> MKQILDSARNYLKNNSRIKTASLISLELPGSTGTSTAFIYLTDYFRDVIYNGILYQAGKVKSISPHKQNRDLSIGSLSFTITGTAQDEVLKLVQNGVSFLDRTVSIHQAIITEDGSILPVDPDTNGPLLYFRGRITGGGIKDNISTSGVGTSTITWNCSNQFYDFDRVNGRYTDDASHRGLEVVAGQLLPSNGAKRLEYQEDYGFFHANKSISILAKYQVQEERYKLKSKKKLFGLSRSYSLKKYYETVTKEVDIDFNLAAKYIPVVYGVQKIPGIPIFADTELHNPNIVYVVYAFAEGEIDGFLDFSFGDNPMICVDANDSSARTCFGTKKIVGDTMQRIASGISSSSPSVHGQEYRYNDGNGDIRIWTYHGKSNQTASDVLVNIARNRGFYLQNMNGNGPEYWDARYKLLDTAYAVVRFTINENRTEIPEVSAEIQGKKVKVYHSDGRVTANSTSLNGIWQTLDYLTSDRYGANITIDQFPLQQLIQEAAILDIIDESYQVSWQPYWRYVGWTNPLAENRQIVQMNTILDTSESVFKNVQGLLESYGGAINNLSGQYRVTVEKYSNTPLEINFLDTYGDLELSDTTGRNKFNSVQASIVDPALSWKTNSITFYNSNYKEQDKNLDKKLQLSFANITNYYTARSFADRELKKSRYSRTLSFSLPYQFIGIEPNDAIAFTYDRYGWDRKYFLVDEVENSREGKINVTLQEYGEDVFINSGQVDNSGNDIPDISNNVLPPRDFKYTPTPGGLVGSIGKNGELSWLPSLTNNVVYYSIVHSGHAEPYIVQQLETNPNERMIQEIIGEPAGLAIFEIRAVDINGRRSSPVTLSIELNSAKNLSVVSNFRVTNTASGDVTEFVGPDVKLAWDRIPEEDIIESIFYTLEIHDPQNRMLRSVRIENQYTYDYLLTYNKADFALQNSDALGINRKLYFRIRAEGDDGEQSVEWASI;>MRLPDPYTNPELSGLGFESVNLIDNDPVIRDELPNGKVNEVKVSAQYWGINISYPELFPDEYSVLDAFILEYKRTGGYIDVILPQYEAFRVRGNTNLVNIPAGQKGSNITMDTQGVLTGIPKPGDLFKLSNHPKVYKITSFNRSGNSWSINVYPDLFITTTGAEKPVFNGILFRTKLMNGDAFGSTLNNNGTYSGISLNLRESL[2x];> MYYSLMRESKVIVEYDGRAFHFDALSNYDVQTSYEEFKTLRRTIHRRTNYADSVINAQTPSSISLAINFSNTLTEANFFEWLGFDRKGNTFLLPLYSNNIEPIMFNIYIVNKDNNCVYFENCYVSTVDFSLDKNIPILNVGIESGKFSEVSTYREAASIIQGEAMSYSPVIVSTNGNILPGLISASLSFQQQCSWREDKSVFDINKIYNNKRAYVNEMNASATISLYYLKRFAGDMVYNIEPETDVPLNIRNNNISIDFPLARISKRLNFSDVYKVEWDIIPTASSDPVRIDFFGEIKND;>MSTENRVIDIVVDEKVPYGLIMQFMDVDDSVYPPSEIPVNLTGYSLRGTIKSSLDENAETLASFTTSIIDAAQGAAAISLSVADVTNIGEKASKERDKYNPRQRFAGYYDILMTRDVIGSEVSSFRIMEGKVYISDGVTQ[4x];>MALKTKIIVQQILNIDDTTTTASKYPKYTVVLGN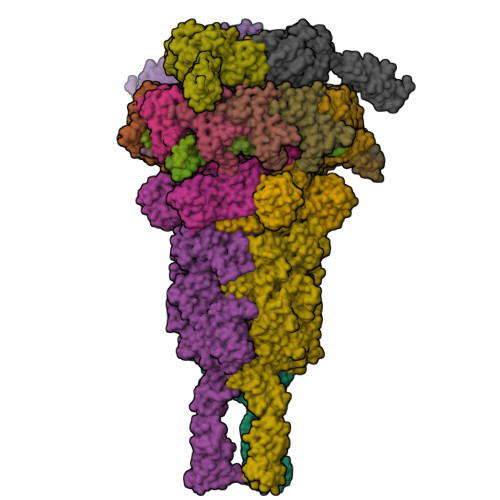SISSITAGELTAAVEASAGSAAAAKGSEIAAKESELNAKDSENEAAISAGASEESASQSAASAAESERQAGLSKGSADNSAASAQESEGFRDSAELAAQNAEQSRLLAEQAKTAAQQAQTAAEAAKTGAETAKDGADAAATTAGEHAAAARQSELNAKISETNAAGSATEAGDKAIDATTEADRAKAEADRATQIVDSKLDKVDISGFIKVYKTKAEADADVVNRVLDEKVLVWNQTNSKYGWYKVAGTAETPVLELVETEQKLTSVNNVRADDAGNVQITLPGGNPSLWLGEVTWFPYDKDSGVGYPGVLPADGREVLRVDYPDTWEAIEAGLIPSVSEAEWQAGASLYFSTGDGSTTFRLPDMMQGQAFRAPTKGEEDAGVIKDQIPYVVTVNGISPDAITGNVEIDTSLQGTVSINQGGTGATTKEDARIALELYSTTEVDSALADKADIATTYTKTEVDSALADKADIATTYTKVEVDSALADAKTQSDTDYLLKANNLSDLADRAAAWLNVRPIGSTPLAGDPVGDYDAVTKRWVENKINTGTVGPTMNGVMNYGVGDFHLRDSRAYIQPYEVVSDGQLLNRADWPELWAYAQMLSPISDADWLADPTKRGQYSLGDGSTTFRVPDRNGVQTGSISALFGRGDGGASSTGGTILDSAAPNITGSFGRLVYASTGTIYEANTGTGAFSAVLSQAKYKRLSEISAADGTAATYPSGFEFFASNSSPVYGRGSTEVRPKAFTGVWVIRASGGFVAANTSWSVINGDATRPADGTTADGGEIISRYNVNGVREAQMSWRIRAQIGAEHYARLNVYNATANRTAVYDFNDLGTFSAENLHSKGAIYSDGNLTIQNQGWPGINFKSNRYNTPATQIGGSTIIEVSGTDGNVSGVNLIRRRGDGNQAGQIIVSFPTTGGAIALQGTSGIEYKKDVTDADAQEAMDRINGQRLVNFVYKDDEQERVRFGVIAEEAELIAPQYIKHNQVSYEDILDEEGNKIGEKTRDRPSVDVNPIVMDLMGCVQALNAKIAALEARIAELESKE[3x];> MTDKLIRELLIDVKQKGATRTAKSIENVSDALENAAAASELTNEQLGKMPKTLYSIERAADRAAKSLTKMQASRGMAGITKSIDSIGAKLDDLSIAMIEVADKLEAGFDGVSRSVKVMGNDVAAATEKVQDRLYDTNRVLGGTARGFNDTAGAAGRASRAIGNTSGSARGATRDFAAMAKVGGGLPLLYAAIASNIFVLQSAFEQLKLGDQLNRLEEFGVIVGTQTGTPVQSLARSLQEAAGYAISFEEAMRQASSASAYGFDAEQLNKFGLVARRAAAVLGVDMTDALNRVIKGVSKQEIELLDELGVTIRLNDAYADYVKQLNAANTGITYNINSLTTFQKQQAYANAVIAESTKRFGYLDEVLRATPWEQFAANADAALRTIQQAAAKYLGPVIDAINTVFYTSQASISAEAARAQEQTNKQIDPTNVGAVALSLSASEEGYNKALDMYKESLDKRNKLKSEFDKRMEQADFYTKLAIRQVGEGIPAGLATAGASEANKKFVEETAAMGLQVARLDKEVTDSTENLNAWKSAYQAAGAAAAKANPEFQKQINLQRDTTDPGAVYDFNSTVLKGLTEQQKAYNQTKKTASDLANDIQNVAQNTDTAAKTSATLADAIKNIESLSLGTGKSADEYVKNLNLGYNTLSEMKTASQALSEYVKLTGNETKNQLAVQQKIADVYNQTKDKEKAQEAGRRLELQQLEEQEAALRRVLQTNQGNKAVEREIEKIQLEKIKLTNQGMEAQKKVKDYTDKILGVDREIALLNNRTMTDTQYRLAQLNLELTIEKEKYEWYTKQADKQKEAEQSRRAQAQIEREIWKFHQDQQAEMTSKRQEAFENTLTSMFPLAGEMQKMEMQLDFYTQMKELTKDNANEQMRWNAEIAKTRAQMSALTAQRNAQMQSSVGSSLGAVYTPTTGLSGEDKKFADMGNQLASYDQAISKLSELNSEATAVAQSMGNLANAMIQFSQGSLDTTSTIAVGMQTVASMIQYSTSQQVSAIDQAIAAEQKRDGKSEASKAKLKKLEAEKLKIQQDAAKKQIIIQTAVAVMQAATAVPYPFSIPLMIAAGLAGALALAQASSASGMSSIGDSGADTASYLTLGERQKNIDVSMSANAGELSYVRGDKGIGNANSFVPRAEGGNMYPGVSYQMGEHGTEVVTPMVPMKATPNDELKNSSNSTAGRPIILNISAMDAASFREFASSNSGALRDAVELALNENGASLKTLGNS;> MSLQLLRNTRIFVSTVKTGHDTTNTQEILVQDDISWGQDSNSTDITVNEAGPRPTRGSKRFNDSLNAAEWSFSTYILPYEDTTTGKQIVPDYMLWHALSSGKAIDLDGDTGAHNNATNFMVNFKDNAYHELAMLHIYILTDNAWSYIDSCQINQAEVNVDIEDIGRVTWSGNGNQLIPLDEQPFDPDALGIDDETYMTIQSSYIKNKLTILKIKDMDSDKEYDIPITGGTFTINNNITYLTPNIMSRVNIPIGSFTGAFELTGSLTAYLNDKSLGSMELYKDLVRTLKVVNRFEIALILGGEYDDERPAAVLVAKQAHVNIPTIETDDVLGTSVEFKAIPTDLDTGDEGYLGFSNKYTKTTVANLIATGDGAETPPILVESITVKSAADATSVTNSDTLQMSVEVTPPEATNTAVTWSISSGDAATIDAESGLLTADVSKTGEVIVKAVAKDGSGVEGTKTITVSAGE> MSNWVMQEENKQGNLTPLFEELLQQCPPGGQNKTAHMVSAYQLAQGNWMPTSCHVFMGTISARRTKTHPYEAYVKLRELVEEHKMKTLCPGSSLGKHNDWIIGKIKYQGNLRTKHMLNPGKVAEQLCREGHRHNVYNKTIGSVMTATGIRLEKLPVVRAQTDTTNFHQAIRDKIDKEENLQTPGLHKKLMEVFNALKRPELESSYDAVEWEELERGINRKGAAGFFERKNIGEILDSEKNKVEEIIDNLKKGRNIKYYETAIPKNEKRDVNDDWTAGDFVDEKKPRVIQYPEAKTRLAITKVMYKWVKQKPVVIPGYEGKTPLFQIFDKVKKEWDQFQNPVAVSFDTKAWDTQVTTKDLELIKDIQKYYFKKKWHKFIDTLTMHMTEVPVICADGEVYIRKGQRGSGQPDTSAGNSMLNVLTMVYAFCEATGVPYKSFDRVAKIHVCGDDGFLITERALGEKFASKGVQILAEAGKPQKITEGDKMKVAYQFDDIEFCSHTPIQVRWSDNTSSYMPGRNTTTILAKMATRLDSSGERGTIAYEKAVAFSFLLMYSWNPLIRRICLLVLSTELQVKPGKSTTYYYEGDPISAYKEVIGHNLFDLKRTSFEKLAKLNLSMSVLGAWTRHTSKRLLQDCVNMGVKEGNWLVNADRLVSSKTGNRYIPGEGHTLQGRG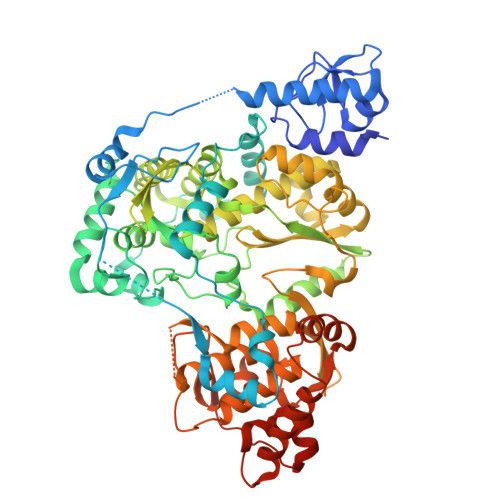SSSHHHHHH> SGIVPTLQNIVATVTLGCRLDLKTVALHARNAEYN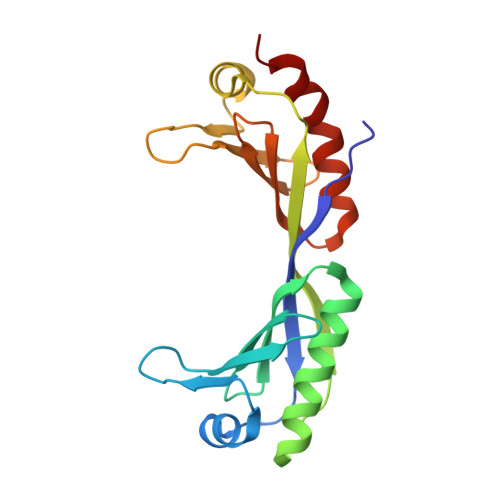PKRFAAVIMRIREPKTTALIFASGKMVVTGAKSEDDSKLASRKYARIIQKIGFAAKFTDFKIQNIVGSCDVKFPIRLEGLAFSHGTFSSYEPELFPGLIYRMVKPKIVLLIFVSGKIVLTGAKQREEIYQAFEAIYPVLSEFRKM>MNHLGKTEVFLNRFALRPLNPEELRPWRLEVVLDPPPGREEVYPLLAQVARRAGGVTVRMGDGLASWSPPEVLVLEGTLARMGQTYAYRLYPKGRRPLDPKDPGERSVLSALARRLLQERLRRLEGVWVEGLAVYRREHARGPGWRVLGGAVLDLWVSDSGAFLLEVDPAYRILCEMSLEAWLAQGHPLPKRVRNAYDRRTWELLRLGEEDPKELPLPGGLSLLDYHASKGRLQGREGGRVAWVADPKDPRKPIPHLTGLLVPVLTLEDLHEEEGSLALS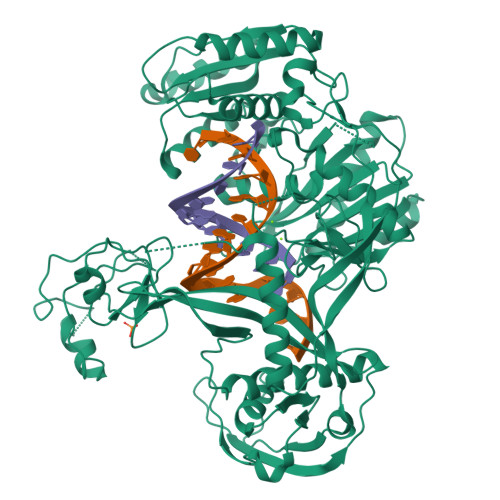LPWEERRRRTREIASWIGRRLGLGTPEAVRAQAYRLSIPKLMGRRAVSKPADALRVGFYRAQETALALLRLDGAQGWPEFLRRALLRAFGASGASLRLHTLHAHPSQGLAFREALRKAKEEGVQAVLVLTPPMAWEDRNRLKALLLREGLPSQILNVPLREEERHRWENALLGLLAKAGLQVVALSGAYPAELAVGFDAGGRESFRFGGAACAVGGDGGHLLWTLPEAQAGERIPQEVVWDLLEETLWAFRRKAGRLPSRVLLLRDGRVPQDEFALALEALAREGIAYDLVSVRKSGGGRVYPVQGRLADGLYVPLEDKTFLLLTVHRDFRGTPRPLKLVHEAGDTPLEALAHQIFHLTRLYPASGFAFPRLPAPLHLADRLVKEVGRLGIRHLKEVDREKLFFV[2x]> MHHHHHHGSM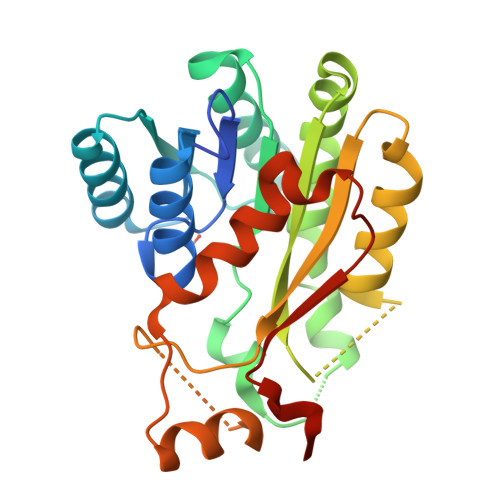GKLDGKVAVVTGGGRGVGRAICVAYAEEGADVVVNYAGNHAAANEVVAMIEKMGRRAVAVQGRVEIKAEAEKTIQTAVDNFGRIDVLVNNAGATKPAMLHKMTEEQWDAVVNIHLKGPFLCVQAAAKYFMEQNYGKIINVTSVAGLVGTTGQINYSAAKGGILSFTMSAARELARFNVTSNVISLGIVTTDMTEKITTDDKLKEIYMRRILLNRYAEPSEVAPAFVFFGCDDSKYITGQLLKVDGGYGLTLQPSLIS>AEKKFLLYDVNFGEGFNLRRDVYMRVANTVRSLRDSGENYILVLPPWGRLHHWKRMEVALSWRLFFDLESLNRFIPVIEFEDFLDENRPIDQVIYLQHYAEGWGTEYVRKFEKRSCLPPAESHYKQVEEFKWKGWFYSYEDVYSRNFQCVSIQGDSGTLKDLLKHSNFSESTSIMVDRAETILHEHYGEVDYWKARRSMRYSNDLVDVADAFRKKYLDSDDKRDKTKLVDDWTKEKPRRTAIGGPYLGIHWRRRDFLYAKKAQLPTIPGTAKILQDLCKKLDLQKIYLATDAPDQEVDELKALLNGELEVYRFTDTQKLNDGQIAIIDQYLCAHAAYFIGSYESTFTFRIQEDREIIGF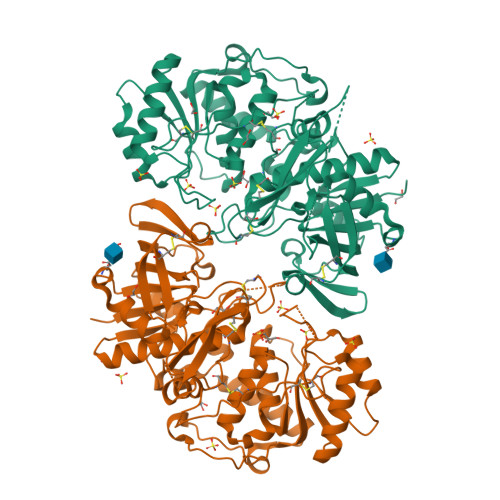PISTTFNRLCPDTEPTCEQPCKWKIVYSSGGGGSGGGGSGGGGGSSGSSIPCLLSPWSCWSDCSVTCGKGMRTRQRMLKSLAELGDCNEDLEQAEKCMLPECP[2x]> I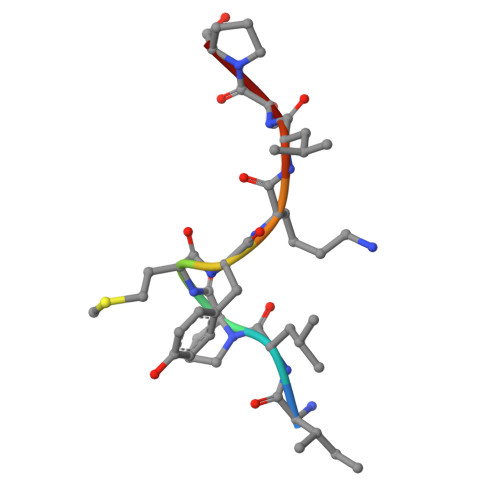LPMYKLSP>[2x]GSPLGQDVFLDYCQKLLEKFRYPWELMPLMYVILKD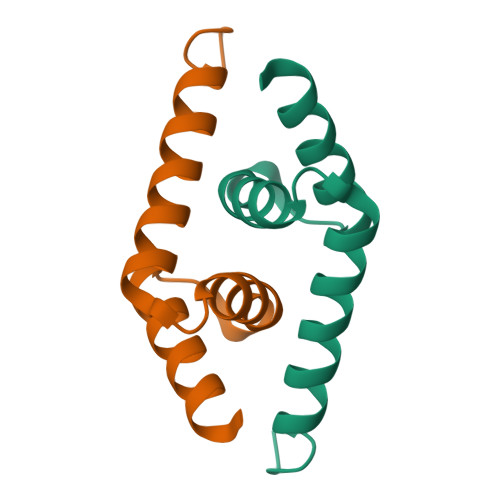ADANIEEASRRIEEGQYVVNEYSRQHNLN> SMIRKQAESYANSTWEVLQYKDSGEPGVLEVFVTINGKVQNITFHIPKTIYMKFKSQTMPLQKIKNCLIEKSSASLPNNPKTSNPAGGQLFKITLPESVFLEEKENCTSIFNDENVLGVFEGTITPHQRAIMDLGASVTFRSKAMGALGKGIQQGFEMKDLSMAENERYLSGFSMDIGYLLHFPTSIGYEFFSLFKSWGDTITILVLKPSNQAQEINASSLGQIYKQMFEKKKGKIETYSYLVDIKEDINFEFVYFTDISKLYRRLSQETTKLKEERGLQFLLLLQSPFITKLLGTIRLLNQMPIVKLSLNEVLLPQLNWQPTLLKKLVNHVLSSGSWISHLIKLSQYSNIPICNLRLDSMDYIIDVLYARKLKKENIVLWWNEKAPLPDHGGIQNDFDLNTSWIMNDSEFPKINNSGVYDNVVLDVGVDNLTVNTILTSALINDAEGSDLVNNNMGIDDKDAVINSPSEFVHDAFSNDALNVLRGMLKEWWDEALKENSTADLLVNSLASWVQNPNAKLFDGLLRYHVHNLTKKALLQLVNEFSALGSTIVYADRNQILIKTNKYSPENCYAYSQYMMKAVRTNPMFSYLDLNIKRYWDLLIWMDKFNFSGLACIEIEEKENQDYTAVSQWQLKKFLSPIYQPEFEDWMMIILDSMLKTKQSYLKLNSGTQRPTQIVNVKKQDKEDSVENSLNGFSHLFSKPLMKRVKKLFKNQQEFILDPQYEADYVIPVLPGSHLNVKNPLLELVKSLCHVMLLSKSTILEIRTLRKELLKIFELREFAKVAEFKDPSLSLVVPDFLCEYCFFISDIDFCKAAPESIFSCVRCHKAFNQVLLQEHLIQKLRSDIESYLIQDLRCSRCHK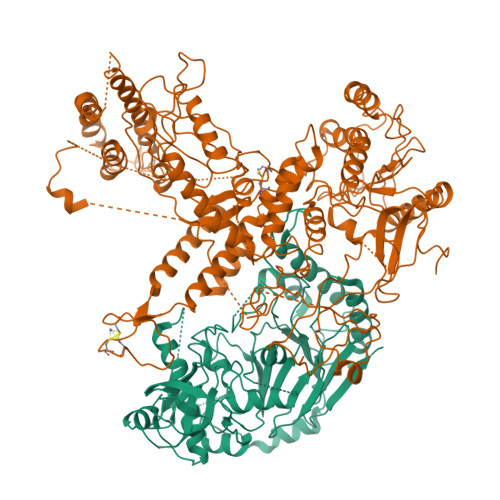VKRDYMSAHCPCAGAWEGTLPRESIVQKLNVFKQVAKYYGFDILLSCIADLT;> MFGSGNVLPVKIQPPLLRPLAYRVLSRKYGLSIKSDGLSALAEFVGTNIGANWRQGPATIKFLEQFAAVWKQQERGLFIDQSGVKEVIQEMKEREKVEWSHEHPIQHEENILGRTDDDENNSDDEMPIAADSSLQNVSLSSPMRQPTERDEYKQPFKPESSKALDWRDYFKVINASQQQRFSYNPHKMQFIFVPNKKQNGLGGIAGFLPDIEDKVQMFLTRYYLTNDRVMRNENFQNSDMFNPLSSMVSLQNELSNTNRQQQSSSNSITPIKNLLGRDAQNFLLLGLLNKNFKGNWSLEDPSGSVEIDISQTIPTQGHYYVPGCMVLVEGIYYSVGNKFHVTSMTLPPGERREITLETIGNLDLLGIHGISNNNFIARLDKDLKIRLHLLEKELTDHKFVILGANLFLDDLKIMTALSKILQKLNDDPPTLLIWQGSFTSVPVFASMSSRNISSSTQFKNNFDALATLLSRFDNLTENTTMIFIPGPNDLWGSMVSLGASGTLPQDPIPSAFTKKINKVCKNVVWSSNPTRIAYLSQEIVIFRDDLSGRFKRHRLEFPFNESEDVYTENDNMMSKDTDIVPIDELVKEPDQLPQKVQETRKLVKTILDQGHLSPFLDSLRPISWDLDHTLTLCPIPSTMVLCDTTSAQFDLTYNGCKVINPGSFIHNRRARYMEYVPSSKKTIQEEIYI> MNLEINNFAPAISSIGSQLCSLSAQKLLTCRKQYGNGAKSFEEFYAEIGGIIGMMGINSQTPSGIREAIYRLYQSAFLFGDIFPESFGIQNTQNIKPPPGFTAPAKKLEVVLPQGGAFDLI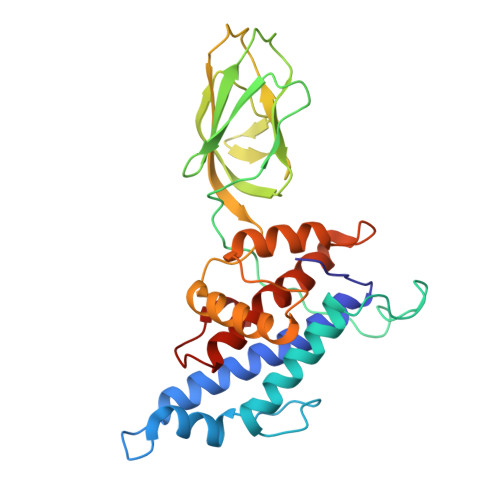YNNGEIRVTTTRNVQAGDLVCTVTFPIQGSVIATRNCHVNEIGGQLTTTRPEIIASVPMPARTVIVASFDAIEIGYGEGDDLFAIGIAILSNRFNGQITPMSRHNYMTQMFANLPANMSERDSSAVLHFAQAAPVVLGMMERLTGAPKWVLDY2-[3-[(1~{R})-1-[(2~{S})-1-[(2~{S})-2-(5-chloranylthiophen-2-yl)-2-cyclohexyl-ethanoyl]piperidin-2-yl]carbonyloxy-3-(3,4-dimethoxyphenyl)propyl]phenoxy]ethanoic 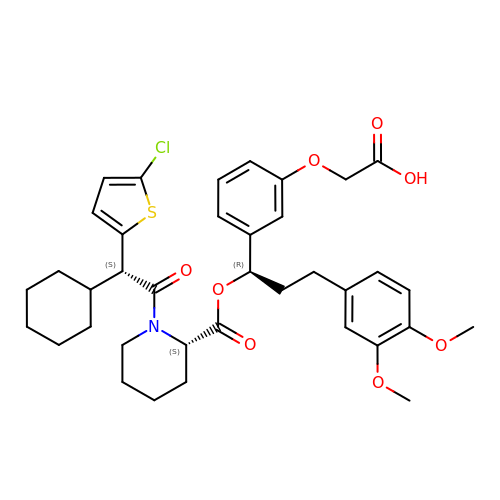acid | C37 H44 Cl N O8 S | GTUUVVDLKBPWFG-JVLQLMMJSA-N> ANPLYQKHIISINDLSRDDLNLVLATAAKLKANPQPELLKHKVIASCFFEASTRTRLSFETSMHRLGASVVGFSDSANTSLGKKGETLADTISVISTYVDAIVMRHPQEGAARLATEFSGNVPVLNAGDGSNQHPTQTLLDLFTIQETQGRLDNLHVAMVGDLKYGRTVHSLTQALAKFDGNRFYFIAPDALAMPQYILDMLDEKGIAWSLHSSIEEVMAEVDILYMTRVQKERLDPSEYANVKAQFVLRASDLH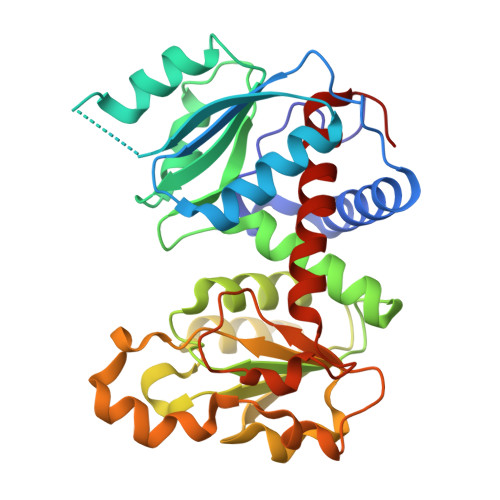NAKANMKVLHPLPRVDEIATDVDKTPHAWYFQQAGNGIFARQALLALVLNRDLVL> TMAASQTSQTVASHVPFADLCSTLERIQKSKGRAEKIRHFREFLDSWRKFHDALHKNHKDVTDSFYPAMRLILPQLERERMAYGIKETMLAKLYIELLNLPRDGKDALKLLNYRTPTGTHGDAGDFAMIAYFVLKPRCLQKGSLTIQQVNDLLDSIASNNSAKRKDLIKKSLLQLITQSSALEQKWLIRMIIKDLKLGVSQQTIFSVFHNDAAELHNVTTDLEKVCRQLHDPSVGLSDISITLFSAFKPMLAAIADIEHIEKDMKHQSFYIETKLDGERMQMHKDGDVYKYFSRNGYNYTDQFGASPTEGSLTPFIHNAFKADIQICILDGEMMAYNPNTQTFMQKGTKFDIKRMVEDSDLQTCYCVFDVLMVNNKKLGHETLRKRYEILSSIFTPIPGRIEIVQKTQAHTKNEVIDALNEAIDKREEGIMVKQPLSIYKPDKRGEGWLKIKPEYVSGLMDELDILIVGGYWGKGSRGGMMSHFLCAVAEKPPPGEKPSVFHTLSRVGSGCTMKELYDLGLKLAKYWKPFHRKAPPSSILCGTEKPEVYIEPCNSVIVQIKAAEIVPSDMYKTGCTLRFPRIEKIRDDKEWHECMTLDDLEQLRGKASGKLASKHLYIGGD

Meanwhile, LigIV catalyzes the ligation step during repair of DSBs through classical nonhomologous end-joining (NHEJ)7 and in V(D)J recombination that is critical for immunoglobulin gene maturation. The mammalian DNA ligases share a conserved catalytic core domain architecture comprised of three subdomains—the DNA-binding (DBD), nucleotidyltransferase (NTD), and oligonucleotide/oligosaccharide-fold (OBD) subdomains. All ligases employ a multi-step catalytic cycle, wherein an active site lysine attacks the α-phosphate moiety of either ATP or NAD+ to form a covalent enzyme-AMP intermediate (Step 1), followed by release of either pyrophosphate (for ATP-dependent ligases) or nicotinamide mononucleotide (for NAD+-dependent ligases). To better understand the unique features of LigIV, we obtained two crystal structures of protein-DNA complexes in the ligation pathway—the lysyl-AMP intermediate in an open conformation, and the DNA–adenylate in a closed conformation.

In order to determine the structural mechanisms underlying LigIV DNA substrate binding, we co-crystallized the LigIV catalytic domain LigIV (Met1-Asp620) in the presence of a nicked duplex DNA substrate containing a 5′-phosphorylated downstream primer and a catalytically incompetent 3′-dideoxycytidine-terminated upstream primer. In a crystallization condition containing 10 mM MgCl2, the enzyme binds the DNA substrate in an open conformation similar to that observed in the previously reported structure without DNA bound (LigIV Met1-Lys609 with bound ATP, PDB ID code 3W5O20, henceforth referred to as the apoprotein). In this open conformation, substrate binding is mediated primarily by the DBD and NTD subdomains, and the OBD does not directly interact with the DNA. First, DBD α-helices 4–6 and α8 engaging the upstream DNA duplex (5′ to the nick) shift by 2.1–3.9 Å to interact with the substrate, while the other DBD secondary structural elements remain comparatively static. In the absence of the DNA substrate, β-strands 6 and 7 are linked by an α-helix (α15) spanning Ile351-Asp357. However, this helix would clash with the upstream duplex when DNA is bound. Thus, this region is displaced and becomes disordered (Lys345-Ser358) upon substrate binding. At 3.25 Å resolution, the electron density for the bound nicked DNA substrate and for the adenylate group covalently linked to the sidechain of Lys273 is clearly defined. In the DNA-bound lysyl-adenylate structure, the nearest 5′-phosphate oxygen on the downstream primer lies ~5.4 Å away from the phosphorus atom of the AMP. Thus, structural repositioning of the 5′-phosphate and/or the lysyl-AMP would be required to facilitate nucleophilic attack and the adenyl-transfer to the DNA.> GMASEFDLIQRYFRRAHPSAVLGVGDDAALIQPSPGMELAVSADMLVANTHFYPNIDPWLIGWKSLAVN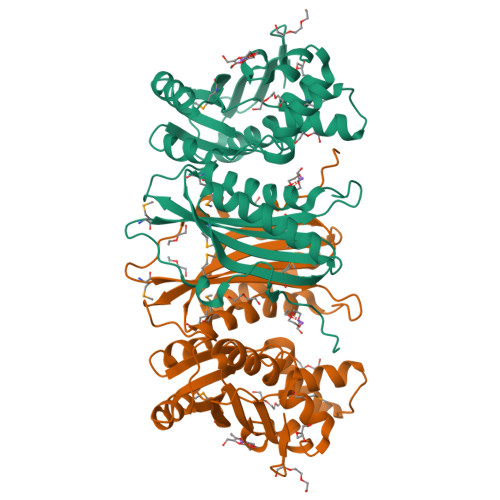ISDMAAMGAQPRWATLTIALPEADEDWISKFAAGFFACAAQFDIALIGGDTTRGPLTISVQIMGETPPGASLLRSTARADDDIWVSGPLGDAALALAAIQGRYPLSDTELAACGKALHQPQPRVVLGQALRGLAHSALDISDGLLADLGHILEHSQVGAEVWLKAIPKSEVVSAHSQEVAIQKMILSGGDDYELCFTASTQHRQQIADIGRQLSLDMAVIGRITDTQQLVIHGLDDAPLTLKEHGFDHFA>[2x]MGSLVCVGTGLQLAGQISVLSRSYIEHADIVFSLLPDGFSQRWLTKLNPNVINLQQFYAQNGEVKNRRDTYEQMVNAILDAVRAGKKTVCALYG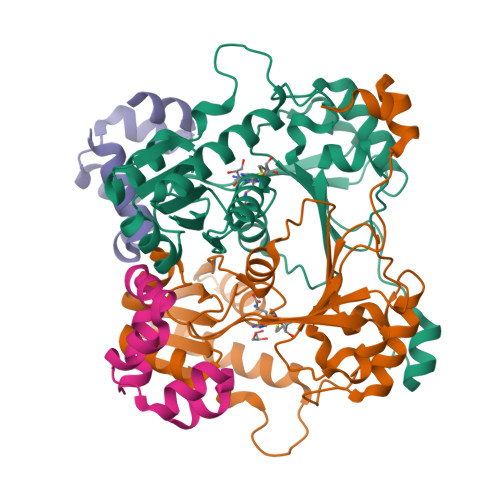HPGVFACVSHMAITRAKAEGFSAKMEPGISAEACLWADLGIDPGNSGHQSFEASQFMFFNHVPDPTTHLLLWQIAIAGEHTLTQFHTSSDRLQILVEQLNQWYPLDHEVVIYEAANLPIQAPRIERLPLANLPQAHLMPISTLLIPPAKKLEYNYAILAKLGIGPEDLG;>[2x]MHHHHHHMSGLSDFFTQLGQDAQLMEDYKQNPEAVMRAHGLTDEQINAVMTGDMEKLKTLSGDSSYQSALVISHGNGD> AETSSATTAQQMPSLAPMLEKVMPSVVSINVEGSTTVNTPRMPRNFQQFFGDDSPFCQEGSPFQSSPFCQGGQGGNGGGQ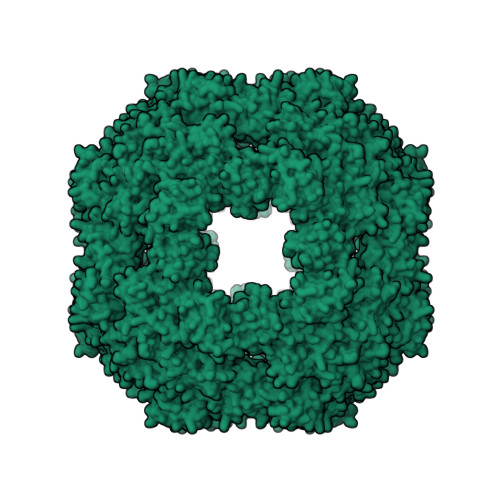QQKFMALGSGVIIDADKGYVVTNNHVVDNATVIKVQLSDGRKFDAKMVGKDPRSDIALIQIQNPKNLTAIKMADSDALRVGDYTVAIGNPFGLGETVTSGIVSALGRSGLNAENYENFIQTDAAINRGNAGGALVNLNGELIGINTAILAPDGGNIGIGFAIPSNMVKNLTSQMVEYGQVKRGELGIMGTELNSELAKAMKVDAQRGAFVSQVLPNSSAAKAGIKAGDVITSLNGKPISSFAALRAQVGTMPVGSKLTLGLLRDGKQVNVNLELQQSSQNQVDSSSIFNGIEGAEMSNKGKDQGVVVNNVKTGTPAAQIGLKKGDVIIGANQQAVKNIAELRKVLDSKPSVLALNIQRGDSTIYLLMQRSHHHHHH> MDPDQYSIEADKKFKYSVKLSDYPTLQDAASAAVDGLLIDRDYNFYGGETVDFGGKVLTIECKAKFIGDGNLIFTKLGKGSRIAGVFMESTTTPWVIKPWTDDNQWLTDAAAVVATLKQSKTDGYQPTVSDYVKFPGIETLLPPNAKGQNITSTLEIRECIGVEV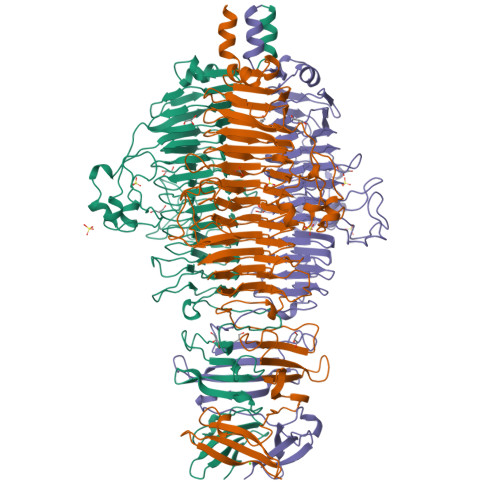HRASGLMAGFLFRGCHFCKMVDANNPSGGKDGIITFENLSGDWGKGNYVIGGRTSYGSVSSAQFLRNNGGFERDGGVIGFTSYRAGESGVKTWQGTVGSTTSRNYNLQFRDSVVIYPVWDGFDLGADTDMNPELDRPGDYPITQYPLHQLPLNHLIDNLLVRGALGVGFGMDGKGMYASNITVEDCAGSGAYLLTHESVFTNIAIIDTNTKDFQANQIYISGACRVNGLRLIGIRSTDGQSLTIDAPNSTVSGITGMVDPSRINVANLAEEGLGNIRANSFGYDSAAIKLRIHKLSKTLDSGALYSHINGGAGSGSAYTQLTAISGSTPDAVSLKVNHKDCRGAEIPFVPDIASDDFIKDSSCFLPYWENNSTSLKALVKKPNGELVRLTLATL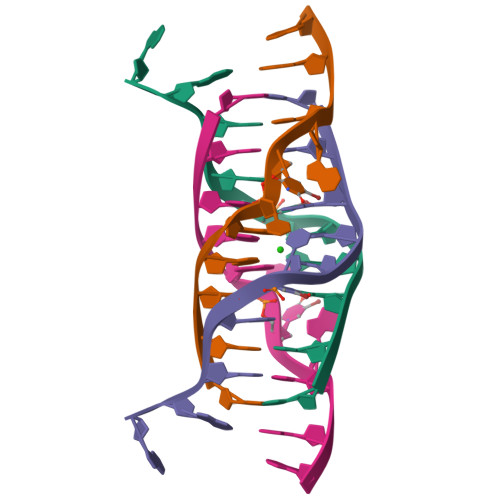>[2x]CCAGGCUGCAA The basil EGS and petunia IGS are closely related to a number of other NADPH-dependent enzymes that act on phenylpropanoid-derived substrates. Structurally, the PIP-family proteins organize around an N-terminal, Rossman-fold domain, containing a core, six-stranded parallel β-sheet flanked on each face by an α-helical layer. In summary, a mechanistic scheme emerges in which binding of the coniferyl acetate substrate within the active site of EGS leads to deprotonation of the p-hydroxy group (PUSH) coupled with expulsion of acetate ion from the C1 substituent (PULL).

The co-crystal structure of EGS complexed with a specifically designed inhibitor, EMDF ((7S,8S)-ethyl (7,8-methylene)-dihydroferulate) provides a view of the substrate-binding mode within the active site of EGS. However, EMDF cannot serve as a substrate of EGS because within the C1 substituent, a cyclopropyl group replaces of the C7-C8 double bond and the orientation of the ester is reversed. A key interaction between EMDF and EGS is the packing of the inhibitor's phenyl ring parallel to the A-face of the cofactor's nicotinamide ring (interplanar separation 3.4 Å). The para-hydroxy group of the inhibitor's guaiacol moiety hydrogen bonds with the backbone amide-nitrogen of Val114 and also interacts via a bridging water molecule with the side-chain amino group of Lys132. The inhibitor's C1 substituent bearing the cyclopropyl and ethyl-ester moieties projects into a cavity formed by the C-terminal domain of the protein. In contrast, the cyclopropyl group of EMDF induces a distinct kink in the conformation of the side group, which steers the end of the side group into a hole formed within the capping region. The stringent binding selectivity of EGS is further emphasized by the observation that only the 7-(S),8-(S) stereoisomer of EMDF complexed with EGS; the 7-(R),8-(R) isomer (present at low levels in the EMDF preparation) was excluded, due to poorer steric complementarity with the EGS active site. Although the binding of EMDF exploits shape features of the EGS active site that are inaccessible to the coniferyl acetate substrate, the structure of the EGS-NADP+-EMDF complex nevertheless provides a useful framework for probing the EGS enzymatic mechanism. The structure of the EGS-NADP+-EMDF complex shows that the ε-amino group of Lys132 forms interactions with both the nicotinamide-ribose of NADP(H), and potentially, the substrate molecule. The Lys132 interaction with the substrate is particularly intriguing, as it is not proximal to the site of hydride addition (as suggested in the case of IFR), but instead involves the p-hydroxyl group via a bridging water molecule.

>[2x]SGHGMEENGMKSKILIFGGTGYIGNHMVKGSLKLGHPTYVFTRPNSSKTTLLDEFQSLGAIIVKGELDEHEKLVELMKKVDVVISALAFPQILDQFKILEAIKVAGNIKRFLPSDFGVEEDRINALPPFEALIERQRMIRRAIEEANIPYTYVSANCFASYFINYLLRPYDPKDEITVYGTGEAKFAMNYEQDIGLYTIKVATDPRALNRVVIYRPSTNIITQLELISRWEKKIGKKFKKIHVPEEEIVALTKELPEPENIPIAILHCLFIDGATMSYDFKENDVEASTLYPELKFTTIDELLDIFVHDPPPPASAAF> MRNLKLHRTLEFRDIQAPGKPQCFCLRAEQGTVLIGSERGLTEVDPVRREVKTEISLVAEGFLPEDGSGCIVGIQDLLDQESVCVATASGDVIVCNLSTQQLECVGSVASGISVMSWSPDQELLLLATAQQTLIMMTKDFEVIAEEQIHQDDFGEGKFVTVGWGSKQTQFHGSEGRPTAFPVQLPENALPWDDRRPHITWRGDGQYFAVSVVCRQTEARKIRVWNREFALQSTSESVPGLGPALAWKPSGSLIASTQDKPNQQDVVFFEKNGLLHGHFTLPFLKDEVKVNDLLWNADSSVLAIWLEDLPKEDSSTLKSYVQLWTVGNYHWYLKQSLPFSTTGKNQIVSLLWDPVTPCRLHVLCTGWRYLCCDWHWTTDRSSGNSANDLANVAVIDGNRVLVTVFRQTVVPPPMCTYRLLIPHPVNQVIFSAHLGNDLAVLDASNQISVYKCGDKPNMDSTVKLGAVGGNGFKVPLTTPHLEKRYSIQFGNNEEEEEEEVNALQLSFLTWVEDDTFLAISYSHSSSQSIIHHLTVTHSEVDEEQGQLDVSSSVTVDGVVIGLCCCSKTKSLAVQLADGQVLKYLWESPSLAVEPWKNSEGIPVRFVHPCTQMEVATIGGEECVLGLTDRCRFFINDTEVASNITSFAVCDDFLLVTTHSHTCQVFSLSGASLKMLQAALSGSHEASGEILRKVERGSRIVTVVPQDTKLILQMPRGNLEVVHHRALVLAQIRKWLDKLMFKEAFECMRKLRINLNLIHDHNPKVFLENVETFVKQIDSVNHINLFFTELREEDVTKTMYPPPITKSVQVSTHPDGKKLDLICDAMRAAMEAINPRKFCLSILTSHVKKTTPELEIVLQKVQELQGNLPFDPESVSVEEALKYLLLLVDVNELFNHSLGTYDFNLVLMVAEKSQKDPKEYLPFLNTLKKMETNYQRFTIDKYLKRYEKALGHLSKCGPEYFTECLNLIKDKNLYKEALKLYRPDSPQYQAVSMAYGEHLMQEHLYEPAGLVFARCGAQEKALEAFLACGSWQQALCVAAQLQMSKDKVAGLARTLAGKLVEQRKHSEAATVLEQYAQDYEEAVLLLLEGSAWEEALRLVYKYDRVDIIETSVKPSILEAQKNYMDFLDSETATFIRHKNRLQVVRALRRQAPQVHVDHEVAHGPESDLFSETSSIMSGSEMSGRYSHSNSRISARSSKN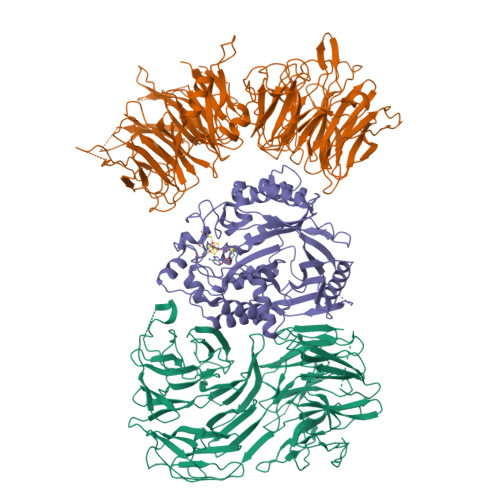RRKAERKKHSLKEGSPLEGLALLEALSEVVQSVEKLKDEVRAILKVLFLFEFEEQAKELQRAFESTLQLMERAVPEIWTPAGQQSSTTPVLGPSSTANSITASYQQQKTCVPALDAGVYMPPKMDPRSQWKLSLLE;> MVSSVLEVSHVFCCPNRVRGALSWNTGPGGLLAFGTSCSVVLYDPQKKVVITNLNGHTARVNCLQWIRTEDGSPSNELVSGGSDNRVIHWELENNQVLKSVRLQGHEGPVCAVHAIYQSGPSEGEQHALIASAASDSTVRIWSKKGSEVKYLQTLSFRDGFVLSVCLAILPGTNVPVLACGDDDCRIHLYIQQDDQFQKALSLCGHEDWIRGVEWATFGRDLFLASCSQDCLIRIWRLYMKPASFETKDGSLRLKENTFTIKDGGVRTTVAVTLETVLAGHENWVNAVHWQPSFYKDGVLQQPVRLLSASMDKTMILWAPDEESGVWLEQVRVGEVGGNTLGFYDCQFGENGTMIIAHAFHGALHLWKQSTVNPRQWAPEIVISGHFDGVQDLMWDPEGEFIITTSTDQTTRLFAPWKKKDQKDRSQVTWHEIARPQIHGYNIKCLAMIDRFQFVSGADEKVLRVFSAPRNFVENFSVISRQSLSHMLCDDQDLPEGATVPALGLSNKALFQGDIASQPFEEDELISPAFGSPQVTFQPAVLNEPPTEDHLLQNTLWPEIQKLYGHGYEIVCVACNNSKTLLASACKASQKEHAAIILWSTASWKQVQSLAFHTLTVTQMTFSPDDKFLLAVSRDRTWSLWKRQDATSSEFDPFFSLFAFTNKITSVHSRIIWSCDWSPDNKYFFTGSRDKKVVVWGECKSSHNPMEHPIRPCSSILDVGSSVTAVSVCPVLNPAQRYIVAIGLESGKICIYSWNKTNQEINDWTSCVETNPSQSHSLGIRRLCWKSCSDDDDDDDDDDTEQSEEGPEWLHFASCGEDHTVKIYRVNRRAL;> MRQKRKGDLSPAELMMLTIGDVIKQLVEAHEQGKDVDLNKMKTKTAAKYGLASQPRLVDIIAAVPPHYRKILIPKLKAKPVRTASGIAVVAVMCKPHRCPHISFTGNICIYCPGGPDSDFEYSTQSYTGYEPTSMRAIRARYDPFLQTRHRIEQLKQLGHSVDKVEFIVMGGTFMALPEEYRDYFIRSLHDALSGHTSNNIHEAIKYSERSFTKCVGITIETRPDYCMKRHLSDMLTYGCTRLEIGVQSVYEDVARDTNRGHTVKAACESFHLAKDSGFKVVTHMMPDLPNVGLERDIEQFIEFFENPAFRPDGLKLYPTLVIRGTGLYELWKSGRYRSYSPSDLIELVARILALVPPWTRVYRVQRDIPMPLVSSGVEHGNLRELAFARMKDLGIQCRDVRTREVGIQEIHHRVRPYQVELVRRDYVANGGWETFLSYEDPDQDILIGLLRLRKCSEETFRFELGGGVSIVRELHVYGSVVPVSSRDPTKFQHQGFGMLLMEEAERIAREEHGSGKMAVISGVGTRNYYRKIGYRLQGPYMVKMLK>[4x]MHHHHHHSSGMSWTVDIPKEVLPDLPPLPEGMQQQFEDTISRDAKQQPTWDRAQAENVRKILESVPPIVVAPEVLELKQKLADVANGKAFLLQGGDCAETFESNTEPHIRANVKTLLQMAVVLTYGASTPVIKMARIAGQYAKPRSSDLDGNGLPNYRGDIVNGVEATPEARRHDPARMIRAYANASAAMNLVRALTSSGTADLYRLSEWNREFVANSPAGARYEALAREIDSGLRFMEACGVSDESLRAADIYCSHEALLVDYERSMLRLATDEEGNEELYDLSAHQLWIGERTRGMDDFHVNFASMISNPIGIKIGPGITPEEAVAYADKLDPNFEPGRLTIVARMGHDKVRSVLPGVIQAVEASGHKVIWQSDPMHGNTFTASNGYKTRHFDKVIDEVQGFFEVHRALGTH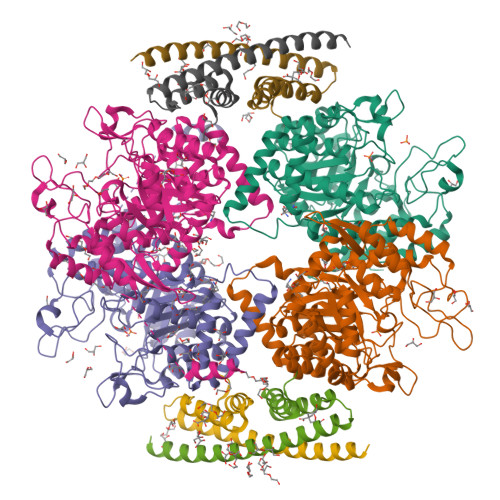PGGIHIEFTGEDVTECLGGAEDITDVDLPGRYESACDPRLNTQQSLELAFLVAEMLRN;>[4x]MPSGTDDPLSDAEIQKYREEINRLDREILDAVKRRTKISQTIGKTRMSSGGTRLVHTREVAIINQFREEIGEEGPALAGILLRMGRGKLG>MTIKVGINGFGRIGRIVFRAAQKRSDIEIVAINDLLDADYMAYMLKYDSTHGRFDGTVEVKDGHLIVNGKKIRVTAERDPANLKWDEVGVDVVAEATGLFLTDETARKHITAGAKKVVMTGP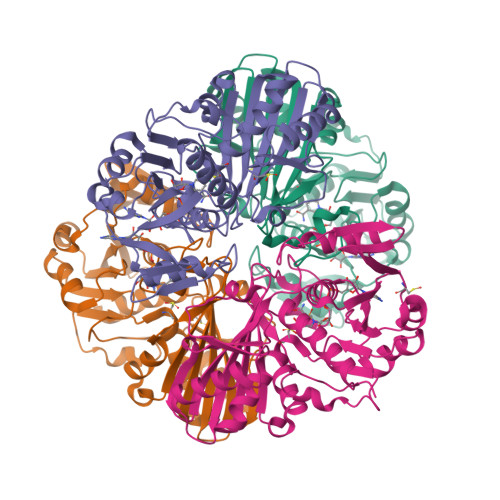SKDNTPMFVKGANFDKYAGQDIVSNASCTTNCLAPLAKVINDNFGIIEGLMTTVHATTATQKTVDGPSHKDWRGGRGASQNIIPSSTGAAKAVGKVLPELNGKLTGMAFRVPTPNVSVVDLTVRLEKAATYEQIKAAVKAAAEGEMKGVLGYTEDDVVSTDFNGEVCTSVFDAKAGIALNDNFVKLVSWYDNETGYSNKVLDLIAHISK[3x];> MVKVGINGFGRIGRLVLRVCMEKGVRVVAVNDPFIDPEYMVYMFKYDSTHGRYKGTVEHKNGRLVVDNLEINVFQCKEPKEIPWSSVGNPYVVEATGVYLSIEAASGHISSGARRVIVTAPSPDAPMLVMGVNEKDYNPGSMTVVSNASCTTNCLAPLAKVIHERFGIVEGLMTTVHAYTATQKTVDGPSKKDWRGGRGAHQNIIPSSTGAAKAVGKVIPELNGKLTGMAFRVPTPNVSVVDLTCRLAQPASYTAIKEAVKAAAKGPMAGILAYTEDQVVSTDFNGDSHSSIFDAKAGIALNDNFVKLVSWYDNEYGYSHRVVDLLRYMFSREK>[2x]MPSSSKSDFSFSTLIIPQHYLRAILKVVSSSSVEVCGFLFGKENRVLKVRFIRNRLNSPVEFEMD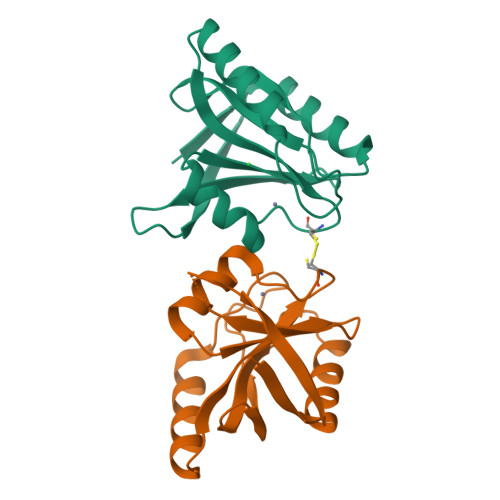PEEMLKALEEAEQENLEVVGIFHSHIACPPIPSGKDLEGMKRWPVIWLIVNEKGEYKAWILSEKNKISEVKIVVE>MKNGRLAGKRVLLTNADAYMGEATVQVFEEEGAEVIADHTDLTKVGAAEEVVERAGHIDVLVANFAVDAHFGVTVLETDEELWQTAYETIVHPLHRICRAVLPQFYERNKGKIVVYGSAAAMRYQEGALAYSTARFAQRGYVTALGPEAARH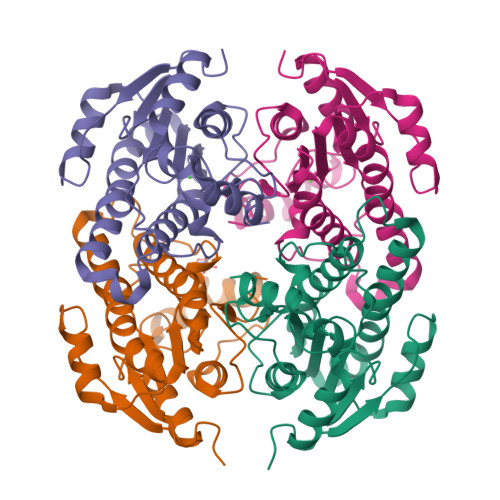NVNVNFIAQHWTQNKEYFWPERIATDEFKEDMARRVPLGRLATAREDALLALFLASDESDFIVGKSIEFDGGWAT[6x]> MGSSHHHHHHSQDPLVPRGSGSDYIIKEKTVLLQKKDSEGFGFVLRGAKAQTPIEEFTPTPAFPALQYLESVDEGGVAWRAGLRMGDFLIEVNGQNVV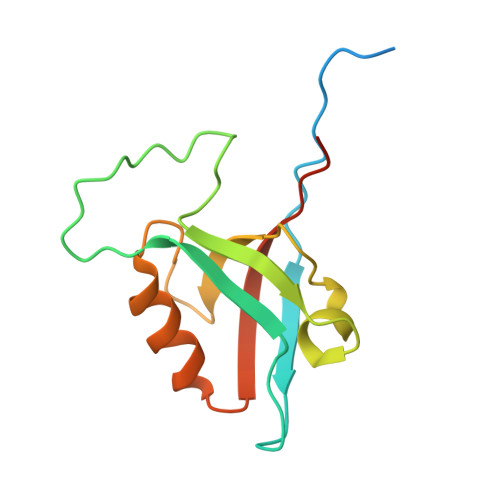KVGHRQVVNMIRQGGNTLMVKVVMVTRHPDMDEA>MHHHHHHSSGR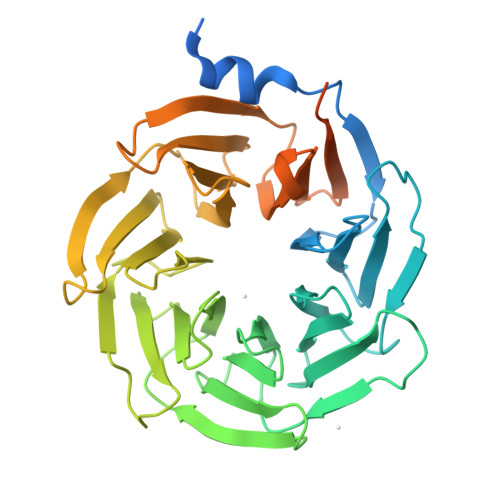ENLYFQGMAGYKPVAIQTYPILGEKITQDTLYWNNYKTPVQIKEFGAVSKVDFSPQPPYNYAVTASSRIHIYGRYSQEPIKTFSRFKDTAYCATFRQDGRLLVAGSEDGGVQLFDISGRAPLRQFEGHTKAVHTVDFTADKYHVVSGADDYTVKLWDIPNSKEILTFKEHSDYVRCGCASKLNPDLFITGSYDHTVKMFDARTSESVLSVEHGQPVESVLLFPSGGLLVSAGGRYVKVWDMLKGGQLLVSLKNHHKTVTCLCLSSSGQRLLSGSLDRKVKVYSTTSYKVVHSFDYAASILSLALAHEDETIVVGMTNGILSVKHRKSEAKKESLPRRRRPAYRTFIKGKNYMKQRDDILINRPAKKHLELYDRDLKH[2x]> MTHQIVTTQYGKVKGTTENGVHKWKGIPYAKPPVGQWRFKAPEPPEVWEDVLDATAYGPICPQPSDLLSLSYTELPRQSEDCLYVNVFAPDTPSQNLPVMVWIHGGAFYLGAGSEPLYDGSKLAAQGEVIVVTLNYRLGPFGFLHLSSFDEAYSDNLGLLDQAAALKWVRENISAFGGDPDNVTVFGESAGGMSIAALLAMPAAKGLFQKAIMESGASRTMTKEQAASTAAAFLQVLGINESQL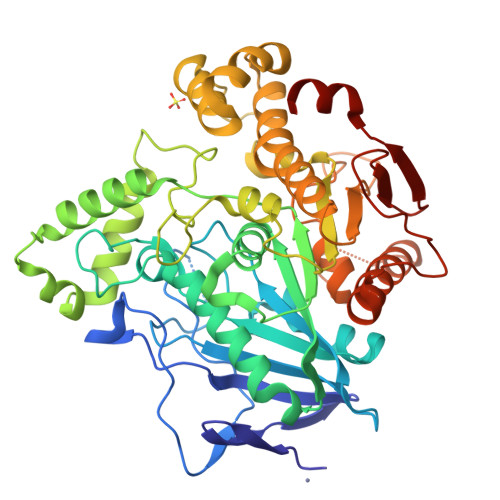DRLHTVAAEDLLKAADQLRIAEKENIFQLFFQPALDPKTLPEEPEKSIAEGAASGIPLLIGTTRDEGYLFFTPDSDVHSQETLDAALEYLLGKPLAEKAADLYPRSLESQIHMMTDLLFWRPAVAYASAQSHYAPVWMYRFDWHPEKPPYNKAFHALELPFVFGNLDGLERMAKAEITDEVKQLSHTIQSAWITFAKTGNPSTEAVNWPAYHEETRETVILDSEITIENDPESEKRQKLFPSKGE We have recently described an additional component in the pantothenate biosynthetic pathway, PanZ, which promotes the activation of the zymogen, PanD, to form aspartate α-decarboxylase (ADC) in a CoA-dependent manner. PanD (encoded by panD) is post-translationally modified to form its catalytically active form, ADC, by cleavage of the peptide backbone between residues Gly24 and Ser25, leading to the formation of a pyruvoyl cofactor from Ser25. The PanD-PanZ protein complex is a cross-shaped heterooctamer, with one PanZ molecule bound to each of the PanD protomer-protomer interfaces. In addition, we show that PanZ acts as a CoA-dependent inhibitor of ADC catalysis.

Bipyrimidal crystals were reproducibly obtained using a 1.1-fold excess of PanZ over PanD(T57V) and a 2-fold excess of AcCoA, with respect to PanZ. X-Ray diffraction data were collected from these crystals to 1.7 Å resolution at room temperature using an in-house X-ray source. The crystals contained a single PanD protomer and one PanZ molecule per asymmetric unit. The structure of the protein complex revealed a highly symmetric heterooctameric complex. The binding site for AcCoA is very close to the protein-protein interface, accounting for the previously observed CoA dependence of the interaction (Monteiro et al., 2012). In particular, binding of AcCoA appears to stabilize the PanZ Leu66-Gly76 loop, which forms contacts with PanD. At the same time, the acetyl portion of the cofactor is held away from PanD on the distal face of PanZ, suggesting that acetylation is not required for activation, consistent with the findings of Stuecker et al. To further investigate how the activation reaction is catalyzed, we compared the structure of the PanD(T57V)-AcCoA.PanZ complex with that of the previously reported structure of the wild-type PanD zymogen in the absence of PanZ (Schmitzberger et al., 2003). The location of the peptide backbone in the immediate region of eventual peptide cleavage (Glu23-Cys26) in the PanD zymogen is largely similar to that observed in the PanD-AcCoA.PanZ complex, although the exact conformations of individual residues, particularly the carbonyl of Gly24, have changed. There is no evidence for ester formation in the structure of PanD(T57V), either alone (Webb et al., 2014) or in complex with PanZ.AcCoA.

> MRGSHHHHHHGLVPRGSMIRTMLQGKLHRVKVTHADLHYEGSCAIDQDFLDAAGILENEAIDIWNVTNGKRFSVYAIAAERGSRIISVNGAAAHCASVGDIVIIASFVTMPDEEARTWRPNVAYFEGDNEMKRTAKAIPVQVA;> MKLTIIRLEKFSDQDRIDLQKIWPEYSPSSLQVDDNHRIYAARFNERLLAAVRVTLSGTEGALDSLRVREVTRRRGVGQYLLEEVLRNNPGVSCWWMADAGVEDRGVMTAFMQALGFTAQQGGWEKCSGLEHHHHHH> GAGCAGACCTG;> ACTGCACTCA;> CAAGT;> TCTGAGTGCGGTCTGC

In this work, we exhaustively probe the ability of all 36 immobile HJ sequences to form DNA crystals in two different designed systems. Three separate self-assembling DNA crystal systems are described in this report: the “4 × 5” and “4 × 6” designs (collectively referred to as the 4 × N systems), and a third construct with a “scrambled” sequence variant of the 4 × 6 lattices. Self-assembly was mediated by three constituent oligonucleotides: (S1) containing four sequence repeats of either 5 or 6 bases; (S2) composed of 21 bases containing complementary regions to both (S1); and (S3) which forms the second junction crossover. The HJ serves as the fundamental component at the core of each unit, and the ultimate assembly of the full lattice is facilitated by the complementary 2-base sticky ends that tail each duplex.

Each asymmetric unit could be defined as either a HJ containing 10 and 11 bp on each arm, or as a 21-bp linear duplex. The 4 × 5 system robustly crystallized with 75% of the junctions, and we obtained crystals in all but 9 of 36 sequences. Pos1 and 2 were readily observable in the electron density maps at either one or both of these conserved sites in a significant number of the structures, with no apparent respect to motif or symmetry. Stereoscopic view, using J21 in the 4 × 5 system, 2Fo–Fc electron density accounting for the bases at the crossover regions are contoured at σ = 2.0, and the individual ion positions 1 and 2 (indicated Pos1 and Pos2) are independently contoured in the corresponding electron density at σ = 4.0. The presence of arsenic at these sites was substantiated by transferring the crystals into TAE-Mg2+ (40 mM Tris, 20 mM acetate, and 1 mM EDTA pH = 8.6), and subsequently freezing the crystals. The crystals were scanned at the arsenic K edge (λ = 1.04 Å) where the corresponding arsenate peak was present. No other components within the crystallization buffers could account for the resulting peaks in the Fo–Fc difference maps for the ions at their corresponding sites. However, in the majority of the crystal structures reported here, the cacodylate anion indeed fits best into the electron density map of our X-ray structures, due to the presence of sodium cacodylate in the crystallization solution.> MESKRNKPGKATGKGKPVGDKWLDDAGKDSGAPIPDRIADKLRDKEFKSFDDFRKAVWEEVSKDPELSKNLNPSNKSSVSKGYSPATP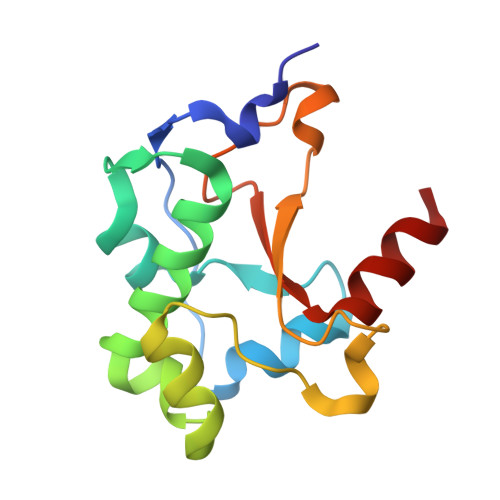KNQQVGGRKVYELHHDKPISQGGEVYDMDNIRVTTPKRHIDIHRGK>[2x]MASAEMRERLEAPLPDRAVPIYVAGFLALYDSGDPGELALDPDTVRAALPPENPLPINVDHRARCEVGRVLAVVNDPRGPFFVGLIACVQLERVLETAASA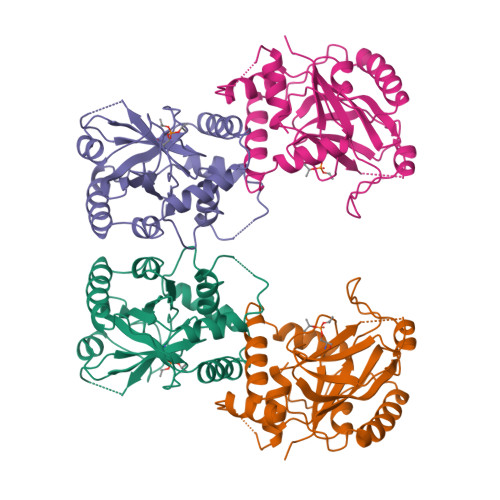AIFERRGPALSREERLLYLITNYLPSVSLSTKRRGDEVPPDRTLFAHVALCAIGRRLGTIVTYDTSLDAAIAPFRHLDPATREGVRREAAEAELALAGRTWAPGVEALTHTLLSTAVNNMMLRDRWSLVAERRRQAGIAGHTYLQA(1R)-3-(3,4-dimethoxyphenyl)-1-{3-[2-(morpholin-4-yl)ethoxy]phenyl}propyl (2S)-1-[(2S,3R)-2-cyclohexyl-3-hydroxybutanoyl]piperidine-2-carboxylate | C39 H56 N2 O8 | 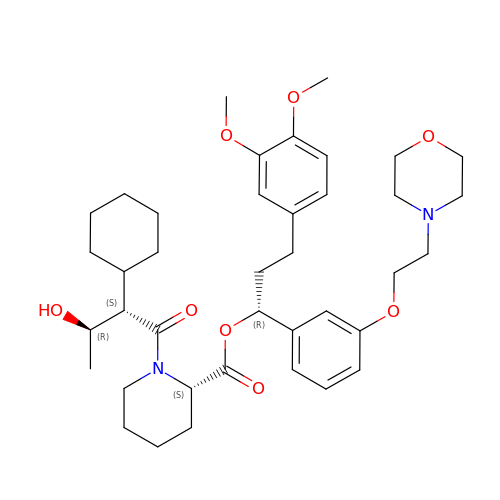RUPZPRKPEAFHDB-JEPHQYQUSA-N> GPHMEDENILRNAVNLQVLKFHYPEIESIIDIASHVAVYQFDVGSQKWLKTSIEGTFFLVKDQRARVGYVILNRNSPENLYLFINHPSNVHLVDRYLIHRTENQHVVGLWMFDPNDMSRIFNIVKESLLR;> MSFTNATFSQVLDDLSARFILNLPAEEQSSVERLCFQIEQAHWFYEDFIRAQNDQLPSLGLRVFSAKLFAHCPLLWKWSKVHEEAFDDFLRYKTRIPVRGAIMLDMSMQQCVLVKGWKASSGWGFPKGKIDKDESDVDCAIREVYEETGFDCSSRINPNEFIDMTIRGQNVRLYIIPGISLDTRFESRTRKEISKIEWHN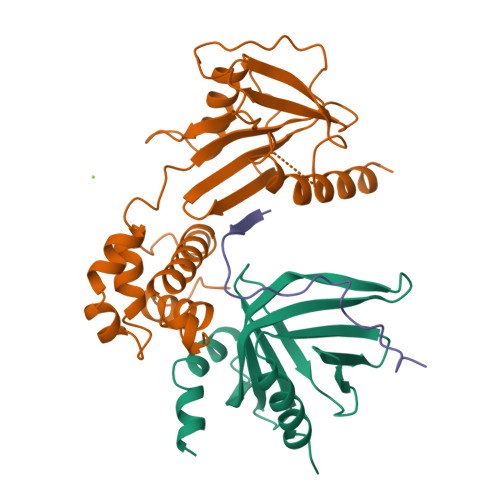LMDLPTFKKNKPQTMKNKFYMVIPFLAPLKKWIKKRNIANNT;> SILYAGPTFTHSPAASNLPIPTFLHS>MEDINWQLFGPNLYTSMVKIAIPDFFERIRVKGDGNCFFRAFAYLFFDTEEMWDTVKGTALGYARQHWSECHGAKGVYNYRAENEIKSEKALYSSVLRGNATENVTRRGLDLYLEDATKEGYWGGTD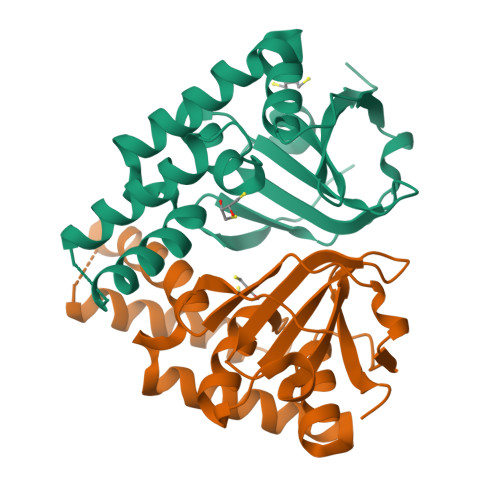EAEMLASALNVTIVIWNVNTDMKVLDVQKFGTDSVPRAFNIVRCGAHFDALKLINQHGTEAATVSTKSGSHHHHHH[2x]>MASMTGGQQMGRGSEEPNPNDGYDYMQHGFDWPGLQEGGTTKYPACSGSNQSPIDINTNQLMEPSSRSGTSAVSLNGLNVDGAQADGITLTNAKVDLEQGMKVTFDQPAANLPTIEIGGTTKSFVPIQFHFHHFLSEHTINGIHYPLELHIVMQEQDPADVATAQLAVIGIMYKYSENGDAFLNSLQTQIEGKIGDGTASYGDTGVSIDNINVKTQLLPSSLKYAGYDGSLTTPGCDERVKWHVFTTPREVTREQMKLFVDVTMGAHAGA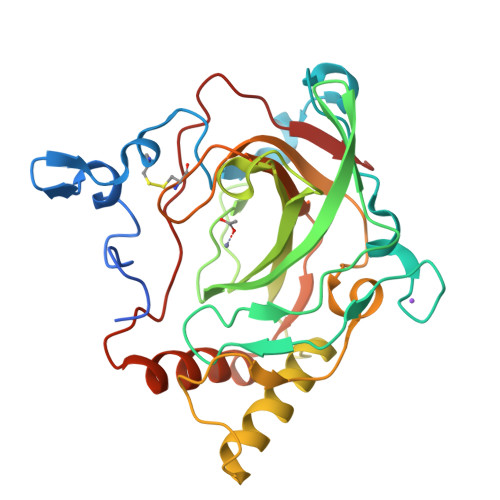DVVNNRMIQDLGDREVYKYNY[2x]> MKFLLAFSLLIPSVVFASSSKFQQVEQDVKAIEVSLSARIGVSVLDTQNGEYWDYNGNQRFPLTSTFKTIACAKLLYDAEQGKVNPNSTVEIKKADLVTYSPVIEKQVGQAITLDDACFATMTTSDNTAANIILSAVGGPKGVTDFLRQIGDKETRLDRIEPDLNEGKLGDLRDTTTPKAIASTLNKFLFGSALSEMNQKKLESWMVNN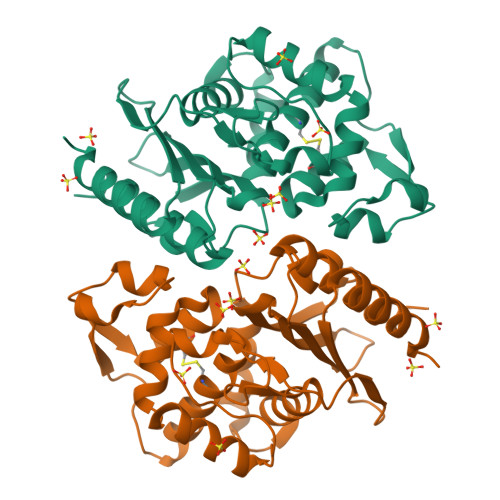QVTGNLLRSVLPAGWNIADRSGAGGFGARSITAVVWSEHQAPIIVSIYLAQTQASMEERNDAIVKIGHSIFDVYTSQSR> AERPTLPIPDLLTTDARNRIQLTIGAGQSTFGGKTATTWGYNGNLLGPAVKLQRGKAVTVDIYNQLTEETTLHWHGLEVPGEVDGGPQGIIPPGGKRSVTLNVDQPAATCWFHPHQHGKTGRQVAMGLAGLVVIEDDEILKLMLPKQWGIDDVPVIVQDKKFSADGQIDYQLDVMTAAVGWFGDTLLTNGAIYPQHAAPRGWLRLRLLNGCNARSLNFATSDNRPLYVIASDGGLLPEPVKVSELPVLMGERFEVLVEVNDNKPFDLVTLPVSQMGMAIAPFDKPHPVMRIQPIAISASGALPDTLSSLPALPSLEGLTVRKLQLSMDPILDMMGMQMLMEKYGDQAMAGMDHSQMTSFAEYWALLSMNHGGKFDFHHANKINGQAFDMNKPMFAAAKGQYERWVISGVGDMMLHPFHIHGTQFRILSENGKPPAAHRAGWKDTVKVEGNVSEVLVKFNHDAPKEHAYMAHCHLLEHEDTGMMLGFTVKDPNSSSVDKLAAALEHHHHH;> GPMSVPTDGAVTTSQIPASEQETLVRPKPLLLKLLKSVGAQKDTYTMKEVL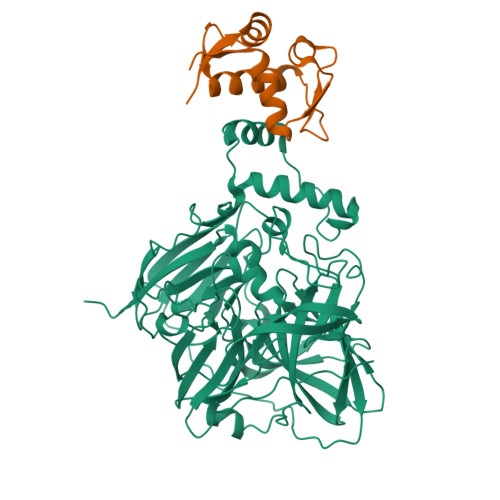FYLGQYIMTKRLYDEKQQHIVYCSNDLLGDLFGVPSFSVKEHRKIYTMIYRNLVVVNQQESSDSGTSVSEN> GAADKGEIRVGNRYQADITDLLKEGEEDGRDQSRLETQVWEAHNPLTDKQIDQFLVVARSVGTFARALDCSSSVRQPSLHMSAAAASRDITLFHAMDTLHKNIYDISKAISALVPQGGPVLCRDEMEEWSASEANLFEEALEKYGKDFTDIQQDFLPWKSLTSIIEYYYMWKTTDRYVQQKRLKAAEAESKLKQV;> MAQTQGTRRKVCYYYDGDVGNYYYGQGHPMKPHRIRMTHNLLLNYGLYRKMEIYRPHKANAEEMTKYHSDDYIKFLRSIRPDNMSEYSKQMQRFNVGEDCPVFDGLFEFCQLSTGGSVASAVKLNKQQTDIAVNWAGGLHHAKKSEASGFCYVNDIVLAILELLKYHQRVLYIDIDIHHGDGVEEAFYTTDRVMTVSFHKYGEYFPGTGDLRDIGAGKGKYYAVNYPLRDGIDDESYEAIFKPVMSKVMEMFQPSAVVLQCGSDSLSGDRLGCFNLTIKGHAKCVEFVKSFNLPMLMLGGGGYTIRNVARCWTYETAVALDTEIPNELPYNDYFEYFGPDFKLHISPSNMTNQNTNEYLEKIKQRLFENLRMLPHA;> LGKGGAXRH

Class I histone deacetylases (HDACs) are enzymes involved in ‘epigenetic' gene regulation through controlling the acetylation state of lysine sidechains in histone tails. They act as the catalytic subunit of several large protein complexes that repress gene expression when targeted to the genome. HDACs 1–3 are assembled into at least five large multi-protein co-repressor complexes that are recruited to chromatin through interaction with repressive transcription factors or other silencing co-factors. Recent structural and functional studies of class I HDACs in complex with their cognate co-repressors have suggested that the activity of these complexes is regulated in the cell by inositol phosphates that are likely derived from membrane phospholipids234.

To understand how a substrate, such as the histone H4 tail, interacts with HDAC1, we synthesized a novel inhibitor based on this peptide. This inhibitor (termed H4K16Hx) comprises residues 12–18 of histone H4 with K16 being replaced by a hydroxamic acid functionality. To investigate this, we soaked crystals of the HDAC1:MTA1 complex (which had been co-crystallized with a peptide-based inhibitor) with 225 mM InsP6 before freezing for data collection. The structure shows that the InsP6 is bound as predicted in the pocket formed at the interface of HDAC1 and MTA1, adjacent to the active site of HDAC1. In particular the inositol ring is tipped away from the HDAC (towards MTA1), which seems to correlate with the sidechain of R270 (HDAC1) adopting a different position from that of the corresponding R265 in HDAC3. The molecule is supported in this new position through a hydrogen bond between the hydroxyl of Y336 and the C3 phosphate group of the InsP6. Careful analysis of the orientation of the InsP6 molecule at the inter-molecular interface showed that the electron density clearly fits best when the inositol phosphate orientation is rotated by 120° relative to that seen in the HDAC3:SMRT:Ins(1,4,5,6)P4 complex. The peptide was observed to be bound at the active site of the enzyme with nearly 100% occupancy, although residues Lys12 and Gly13 were not observed in the electron-density map suggesting that these are not constrained on substrate binding. Several backbone amides in the H4K16 peptide make complementary polar contacts with the sidechain of D99 at the rim of the HDAC active site. Comparison with the structure in the absence of the histone peptide suggests that this residue, and its immediate neighbours, undergo a conformation change on peptide binding.>MGSSHHHHHHSAALEVLFQGPDYKFWYTQPVPKINDEFNESVNEPFISDNKVEDVRKDEYKLPPGYSWYVCDVKDEKDRSEIYTLLTDNYVEDDDNIFRFNYSAEFLLWALTSPNYLKTWHIGVKYDASNKLIGFISAIPTDICIHKRTIKMAEVNFLCVHKTLRSKRLAPVLIKEITRRINLENIWQAIYTAGVYLPKPVSDARYYHRSINVKKLIEIGFSSLNSRLTMSRAIKLYRVEDTLNIKNMRLMKKKDVEGVHKLLGSYLEQFNLYAVFTKEEIAHWFLPIENVIYTYVNEENGKIKDMISFYSLPSQILGNDK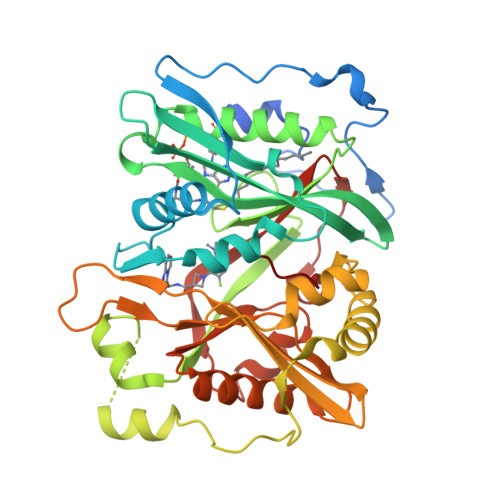YSTLNAAYSFYNVTTTATFKQLMQDAILLAKRNNFDVFNALEVMQNKSVFEDLKFGEGDGSLKYYLYNWKCASFAPAHVGIVLL[2x]> SM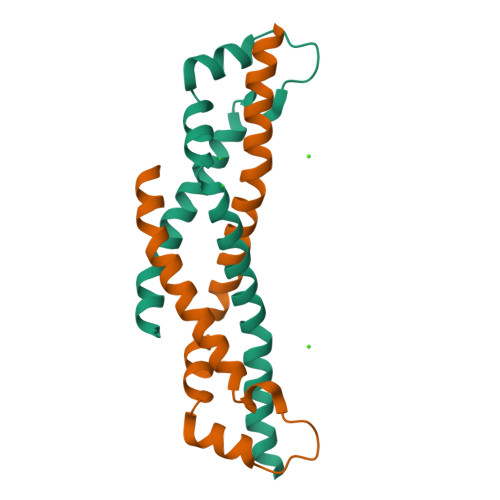KQDQLIVEKMEQTYEAFSPKLANLIEALDAFKEHYEEYATLRNFYSSDEWFRLANQPWDDIPSGVLSEDLLFDMIGDHNQLAADIADLAPIMAKHM> MTWKCNLCGYENDDDALFCIKCGAQKSSEAQQLPQQQPSEPQAQGVVTQQQVVTNPPVQAQVAT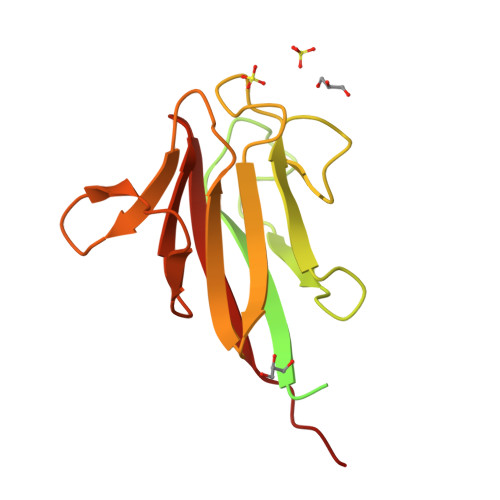PQQPAQQPVLPQPEPAQPQPVSSTPAPQQASQPTNRYYIYFIQTPNENLVNKKVLLNFDLFPSVSMGRSPENIVIVPDSEVSRKHAVIYLDNSELYIEDLNSTNGTYVYDGKQFTPIKGKQKIEPNSIIKLGNQTIVRILKEWSHPQFEK>AEAGITGTWYNQLGSTFIVTAGADGALTGTYESAVGNAESRYVLTGRYDSAPATDGSGTALGWTVAWKNNYRNAHSATTWSGQYVGGAEARINTQWLLTSGTTEANAWKSTLVGHATFTKVKP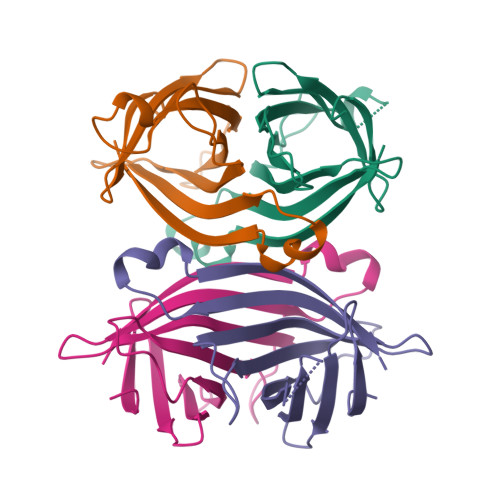SAAS[4x]> MGSSHHHHHHSSGENLYFQGHMSAADTAEDLPEQFRIRRDKRARLLAQGRDPYPVAVPRTHTLAEVRAAHPDLPIDTATEDIVGVAGRVIFARNSGKLCFATLQDGDGTQLQVMISLDKVGQAALDAWKADVDLGDIVYVHGAVISSRRGELSVLADCWRIAAKSLRPLPVAHKEMSEESRVRQRYVDLIVRPEARAVARLRIAVVRAIRTALQRRGFLEVETPVLQTLAGGAAARPFATHSNALDIDLYLRIAPELFLKRCIVGGFDKVFELNRVFRNEGADSTHSPEFSMLET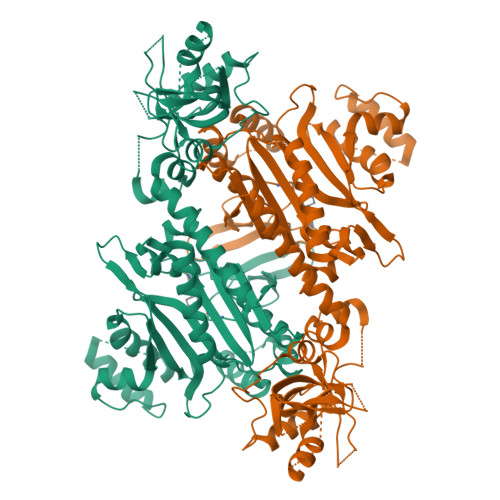YQTYGTYDDSAVVTRELIQEVADEAIGTRQLPLPDGSVYDIDGEWATIQMYPSLSVALGEEITPQTTVDRLRGIADSLGLEKDPAIHDNRGFGHGKLIEELWERTVGKSLSAPTFVKDFPVQTTPLTRQHRSIPGVTEKWDLYLRGIELATGYSELSDPVVQRERFADQARAAAAGDDEAAVLDEDFLAALEYGMPPCTGTGMGIDRLLMSLTGLSIRETVLFPIVRPHSN NRP1 and NRP2 are histone H2A-H2B interacting proteins, closely related to animal SET/TAF-1β and are involved in functions such as histone chaperoning, protein phosphatase 2A (PP2A) inhibition, cell cycle regulation, root meristem formation, heat tolerance, protection of cells from DNA damage during genotoxic stresses, and nucleosome assembly activity in vitro. Here we report the crystal structure of AtNRP2, which reveals a fold similar to that of NAP family proteins, with minor differences as compared to AtNRP1 and SET/TAF-1β. Interestingly, we find that binding affinity to histone H2A-H2B is significantly higher for AtNRP2 than for AtNRP1. We also show that both AtNRP1 and AtNRP2 are capable of nucleosome assembly activity in vitro and thus act as histone chaperones.

Based on this prediction and further alignment with the sequences of AtNRP1 and HsSET/TAF-1β for which crystal structures are known, we decided to truncate the first 13 residues from the N-terminus and 35 residues from the C-terminus of AtNRP2. AtNRP2 NT/CT was heated at 40 °C for 10 min and centrifuged at 13,000× g for 20 min at room temperature before crystallization screening. However, we were able to solve the structure of AtNRP2 NT/CT to a resolution of 3.42 Å in the space group H32 by molecular replacement (MR) method. The overall structure of AtNRP2 revealed an ellipsoid homodimer with a pseudo-two-fold axis, running perpendicular to the long dimerization helix, giving it an earmuff shape. Each monomer could be divided into two domains similar to ScNAP1 and AtNRP1; domain I, which is the dimerization domain and domain II which is the histone-interacting domain. The domain I consist of long antiparallel α-helices of the two monomers arranged in a “tram-track” fashion, which is the characteristic feature of all the NAP family proteins. The dome-shaped structure of AtNRP2 shows an uneven distribution of charge, where the concave face is more acidic in comparison to the convex face of the dimer. The offset in the dimerization domain leads to differences in the end-to-end distance of the curved cleft, and thus AtNRP2 is more curved than AtNRP1. AtNRP2 forms a tetramer assembly with its nearest neighbor. The underside of the earmuff domain is thought to contribute to histone interaction, and as the same region is blocked in the tetramer conformation, it appears that the tetramer assembly (if any) would occlude histone-binding or could probably be a means to regulate histone interaction.

>GPLGSENVEQIDAELVLSIEKLQEIQDDLEKINEKASDEVLEVEQKYNVIRKPVYDKRNEIIKTIPDFWLTAFLSHPALGELLTEEDQKIFKYLSSLDVEDAKDVKSGYSITFSFNPNPFFEDGKLTKTFTFLEEGTTKITATPIKWKEGKGLANGVNHEKNGNKRALPEESFFTWFSDAQHKEDVEDEMQDEQVADIIKEDLWPNPLTYFNNDA[2x]> GSHMSVDLDPSARFAEYAHPERLVSTEWLA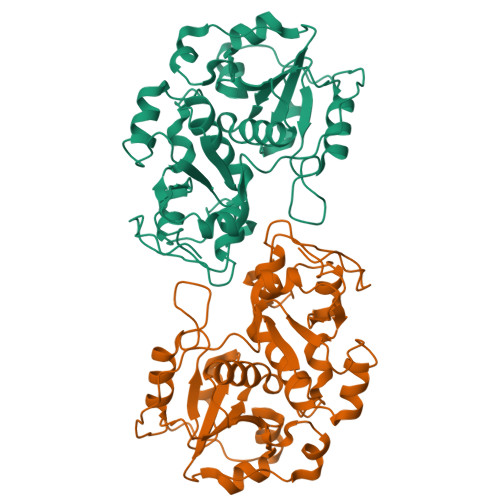AHLGDEGLVVVESDEDVLLYETGHIPGAVKVDWHTDLNDPVQRDYIDGAAFAALLGERGISRDTTVVIYGDKNNWWAAYALWVFTLFGHDDVRLLDGGRSKWEAEGRAYTTDAPTVAATSYPVVERDDSRIRAYRDDVLAHFGKPLIDVRSPEEFSGARTTAPAYPEEGALRAGHIPSAQNVPWGKAAAEDGTFRTLAELDALYRDGAGLKDGDDVVAYCRIGERSSHTWFVLQHLLGFENVRNYDGSWTEWGSAVRVPIVQGSEPGEAPAPIVGR>[2x]AMNTVLELQKLAHD;>NMLYHRYLKPNSEYYKKIEVRGKDNIYELNDIPDTYAVFLDNESVWKHYHVKGSTLPEQGWKIHVTSSLEDSKDVLDKVARLCIDKKIEFKHLKDKDSFMKMNSKNANRASSGKFITIYPTNNEVFVELLEMISLAIQDFKKGPYILNDKRWKNSNVFYRYGGFKGIFNEHGEHCIRDKEGNLIKDQRNPFYQVPDFVKDFDDYLNTINNSGELENKGESRLGKYKIETALSFSNAGGVYLATRKKDNLKVIIKEARPSAGLDGA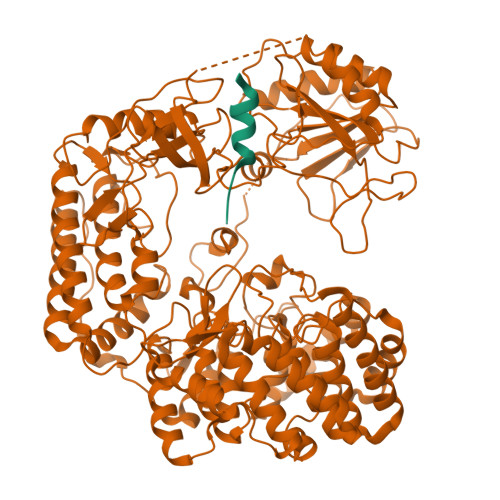AQDALARQKIEYDALKKLKDVSGVVNLIEYFQEWEHYFLVEEFIEGRDLRQWIAQEFPFFEDNNGMSNHIKDVKMILLQLLDLIDSMHNQGVAMGDLQPANIMVTEDLTVRIIDFETAMPVNSDDRPAMLTTGFVSHEMKVSGARDWFGFKRLVRYLALPVLTSEDLEGYLQYNHLNWIKENYGYEFYSFIVDLQEKCDKRIKDYQTFIPKEINLNDQTSDFNLTSIINKLIIGVESSLTNDERFINGDIRQFEMNGGKFNFLTGGSGAAFTLTKNKSSIAEVDKWIQSVLLDNLPLIEEDGLFTGKTGILALLYDKGYKEVVLNELKILKDNINQTDISIRSGLSGIGLFVISLYLETENKEYLKLAKDLERMIKLNRAKDKQLKVKDWMAVDIGVIDGLSGVSLFYSALYSVTQNQKYLEEAEVLIKEDLESTKKDDVTGVLQTVDNKNRLLPYLSGGSIGVAISIWFLNHVSGQDLYREEMNSILKLSKTRCTISGGLFDGAGSFLLIPSMVKNDKNREVILNEVLNLLNIFLIEKNSYYVYPGQFSYRLADDVYTGSSGIILALMGVIKGNPLYWLPLVNSDEFLARTKV[2x]> YNRMKLMIVGNTGSGKTTLLQQLMKTKKSDLGMQSATVGIDVKDWPIQIRDKRKRDL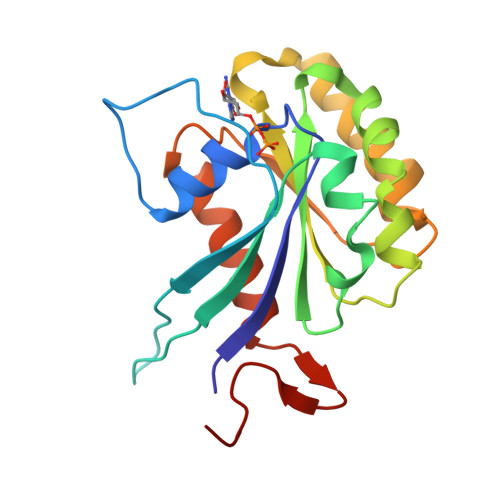VLNVWDFAGREEFYSTHPHFMTQRALYLAVYDLSKGQAEVDAMKPWLFNIKARASSSPVILVGTHLDVSDEKQRKACMSKITKELLNKRGFPAIRDYHFVNATEESDALAKLRKTIINESLNFKIRDQLVVGQLIPD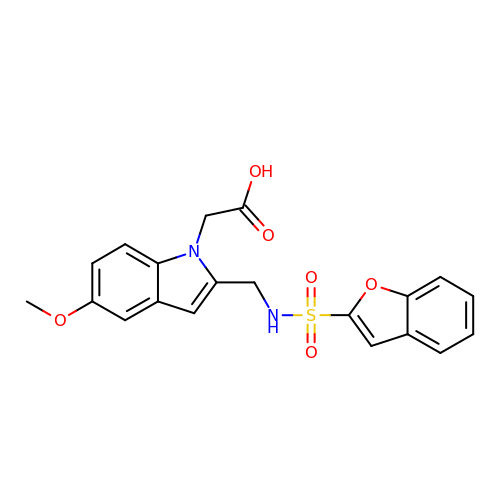(2-{[(1-benzofuran-2-ylsulfonyl)amino]methyl}-5-methoxy-1H-indol-1-yl)acetic acid | C20 H18 N2 O6 S | WZHKFPDZEVEAJG-UHFFFAOYSA-N>[2x]GMPVKKLKQFLDSHKIKYLSIAHSPAYTAQEIAASAHVSGKQLAKTVIIKMDGRLAMVVLPASDHITFMKLKEAIGTSDLELATESEFEGKFAECDVGAMPPFGNL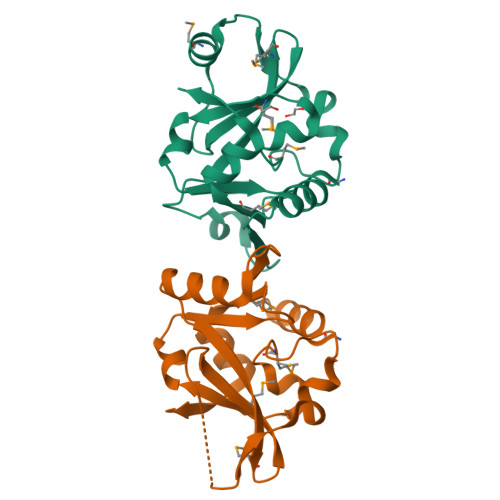YGLPVLVSTKLSAQDNILFNAGSHSELMQLSFGDFEKLVKPTLVTL yersiniabactin 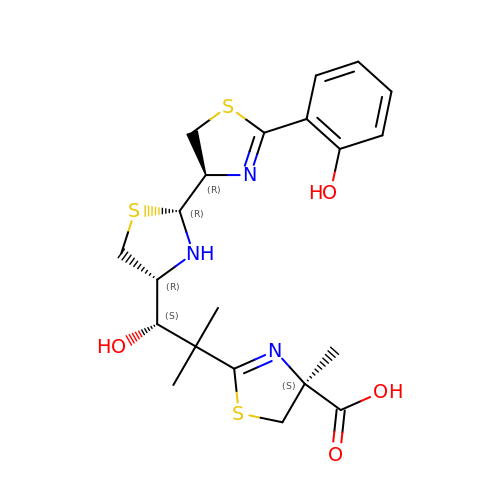| C21 H27 N3 O4 S3 | JHYVWAMMAMCUIR-NIJJZIDKSA-N> MADNQQRCELKLIASPGSWRLYSARKIDERFKSYEQKIFQRDRYTCQFCGFQARLYQDIVNLDGDYTNNRLSNLVTACCFCAQCFFVESVGVGGYGGGTLIYLPELTQAELNSLCHVLFCAITNDTGYKSSAQNIYRSFKFRSQIVEEKFGE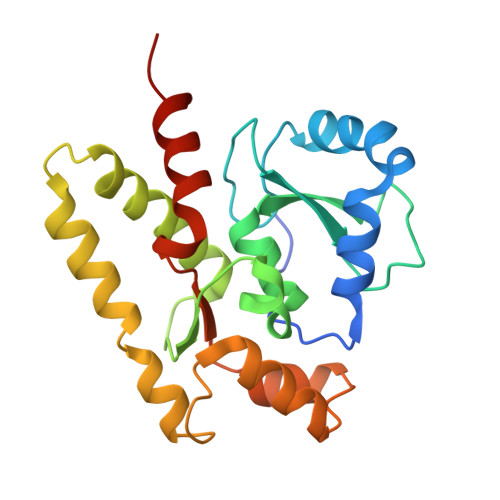GTSDPAIFGQLMIDSGVNSEEIREKLFKNIRLLPSRAKFRKQIEKWAASALEEIAD>MNQQGFVISNELRQQQSELTSTWDLMLQTRINLSRSAARMMMDASNQQSSAKTDLLQNAKTTLAQAAAHYANFKNMTP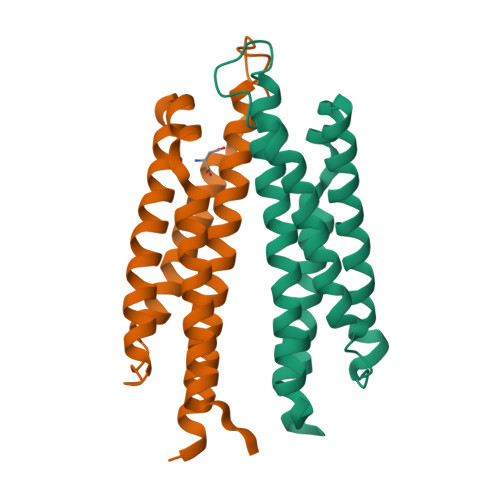LPAMAEASANVDEKYQRYQAALAELIQFLDNGNMDAYFAQPTQGMQNALGEALGNYARVSENLYRQTF[2x]However, a dormant state in Firmicutes can be recapitulated in the laboratory. This paper describes the first structure of a group of peptidoglycan cleaving enzymes from Firmicutes, called stationary phase survival proteins (Sps), that are involved in survival in the stationary phase and are analogous to the resuscitation promoting factors (Rpfs) from Actinobacteria. In this paper we present three high-resolution crystal structures of YuiC, an Sps protein from B. subtilis. The overall fold of each domain of the symmetric dimer consists of a mixed direction six stranded double psi beta barrel surround by five helices. In all the structures, the final two helices and the last strand of the beta barrel of each half are supplied by the other chain in the dimer.

Incubation of YuiC with 5 mM penta-NAG in the crystallisation results in two linked sugars in the final structure per chain. One of the sugars is a NAG that occupies the same −2 site as the sugar in the crystals grown in the presence of NAG monomer. The second sugar has clearly formed a 1,6-anhydro reaction product. The anhydro sugar lies at the −1 position and the unmodified NAG lies at the −2 position in the disaccharide reaction product. NAM can easily be accommodated at the −1 position as the O3 of the sugar, which has the lactic acid group in NAM and then the peptide in peptidoglycan, is pointing into the solvent. The carbonyl oxygen of the acetyl group of the −1 sugar in the YuiC + anhydro product interacts with two main chain NH groups (S154 and A155), which are conserved in MltA (G300 and A301), although the carbonyl also interacts with the side chain OH of S154 in YuiC, which is an extra interaction compared to MltA. The main chain carboxyl of S99 is hydrogen bonding to the N of the N-acetyl group of the −1 anhydrosugar with the side chain of E98 pointing away towards the side chain of T94. However in YuiC the −1 sugar N-acetyl group oxygen of the anhydro product is interacting with S154 and is on the same face as the O6 oxygen would be. Careful inspection of the −3 site indicate some waters are in positions likely to be where hydroxyls of the sugar would be positioned, but if it is present the sugar is either much more mobile or much less occupied due to cleavage at a mixture of positions in the penta-NAG. It is more likely that multiple cleavage events before crystals formed have led to a predominant two sugar anhydro product and this form bound to the dimer may have been preferentially selected by the lattice. We have also trapped an 1,6-anhydrosugar product in the active site, showing that formation of a 1,6-anhydrosaccharide is the product of the reaction.

>[2x]RLKALQQKQTQTTSAAEDKTKPLEEAFDWDEYPVQRVTATGYTAGAESTGKNPGDPLYGLTYSGVKVKRDLYSTVAADPSVFPIGTILFIPNYGLGVVADTGSAIKGNRLDLYFETVKDVYNEWGKKTLDVYVIKKGTGKITEDELEKLNETKSLQVFRNQYKTVK>MRKKPLTIFSDGTLTRRENTLYFESAKGRKPLAIEGIYDIYIYGHVNITSQALHYIAQKGILIHFFNHYGYYDGTFYPRETLLSGDLIIRQAEHYLNKEKRLFLAKSFVTGGTKNMERNLKNWGIKAKLSDYLDELNDARKITEIMNVEARIRQEYYAKWDENLPEEFKIVKRTRRPPKNEMNALISFLNSRLYATIITEIYNTQLAPTISYLHEPSERRFSLSLDLSEIFKPIIADRVANRLVKKGSLKKEHFREDLNGVLLTEEGMKIVTKAYNEELQKSVKHPKI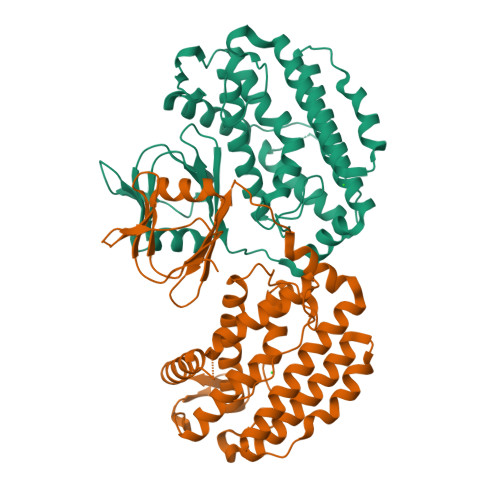GSNVTRQRLIRLEAYKLIKHLVGVEEYKPLVAWF[2x]>[5x]INAEKPNVRFKDMAGNEEAKEEVVEIVDFLKYPERYANLGAKIPKGVLLVGPPGTGKTLLAKAVAGEAHVPFFSMGGSSFIEMFVGLGASRVRDLFETAKKQAPSIIFIDEIDAIGKSRAAGGVVSGNDEREQTLNQLLAEMDGFGSENAPVIVLAATNRPEILDPALMRPGRFDRQVLVDKPD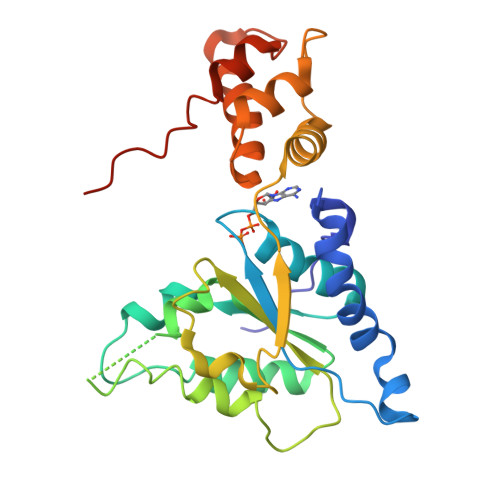FNGRVEILKVHIKGVKLANDVNLQEVAKLTAGLAGADLANIINEAALLAGRNNQKEVRQQHLKEAVERGIAGLEKKLEHHHHHH>[2x]MAHHHHHHMAITLPKLKYALNALSPHISEETL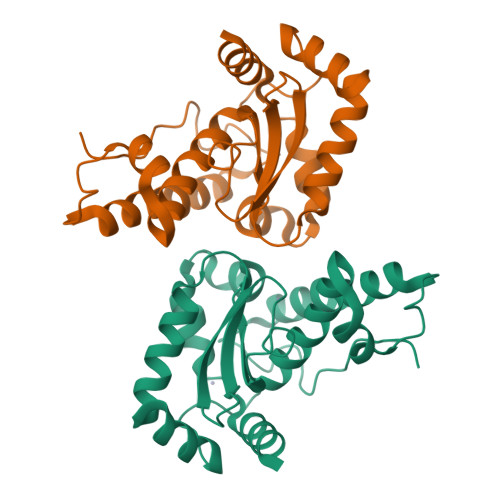SFHYNKHHAGYVNKLNGLIKDTPLANKSLTDILKESTGAIFNNAAQIWNHSFYWDSMGPNCGGEPHGEIKEKIQEDFGSFNNFKDQFSNVLCGHFGSGWGWLALNKNNKLVILQTHDAGNPIKENTGIPILTCDVWEHAYYIDYRNDRLSYVKAWWNLVNWNFANENLKNALNK> GSGELTPGISALEYYERRIRLAETLPPKSCVILAGNDIQFASGAVFYPFQQENDLFYLSGWNEPNSVMILEKPTDSLSDTIFHMLVPPKDAFAEKWEGFRSGVYGVQEIFNADESASINDLSKYLPKIINRNEFIYFDMLSTSNPSSSNFKHIKSLLDGSGNSNRSLNSIANKTIKPISKRIAEFRKIKSPQELRIMRRAGQISGRSFNQAFAKRFRNERTLDSFLHYKFISGGCDKDAYIPVVATGSNSLCIHYTRNDDVMFDDEMVLVDAAGSLGGYCADISRTWPNSGKFTDAQRDLYEAVLNV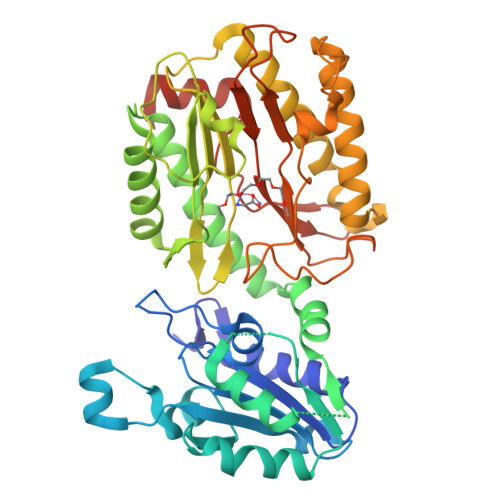QRDCIKLCKASNNYSLHDIHEKSITLMKQELKNLGIDKVSGWNVEKLYPHYIGHNLGLDVHDVPKVSRYEPLKVGQVITIEPGLYIPNEESFPSYFRNVGIRIEDDIAIGEDTYTNLTVEAVKEIDDLENVMQNGLSTKFEEDQVAPL>GMSGQKPVKPSADGLLASARAIKSKGPAPVHLWNPPFNGDIDMRIARDGTWFYQGTPINRPAMVRLFSSILKREEDRFYLVTPVEKVGIRVDDAPFVAVDVEVAGQGRKQVLTFTTHVGDSAVAGEGNPIRMAQDPATGEPAPYVHVRAG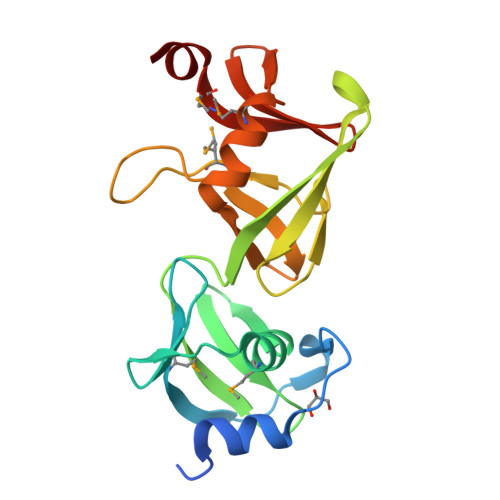LEALIDRKSFYRLMDLGEIEDGWFGLWSSGSFFPLMTVEELERG[2x]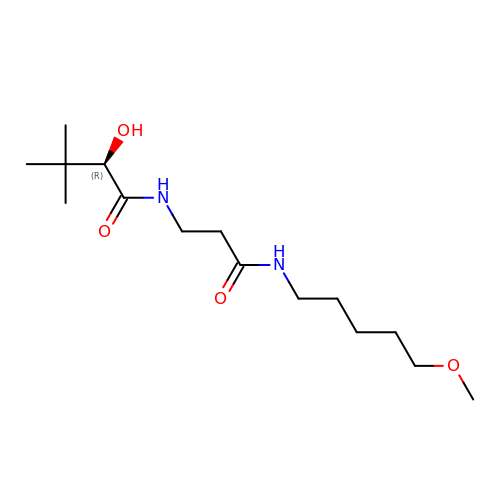(2R)-2-hydroxy-N-{3-[(5-methoxypentyl)amino]-3-oxopropyl}-3,3-dimethylbutanamide | C15 H30 N2 O4 | NABPYAZEODOCAF-ZDUSSCGKSA-N> MLELLPTAVEGVSQAQITGRPEWIWLALGTALMGLGTLYFLVKGMGVSDPDAKKFYAITTLVPAIAFTMYLSMLLGYGLTMVPFGGEQNPIYWARYADWLFTTPLALLDL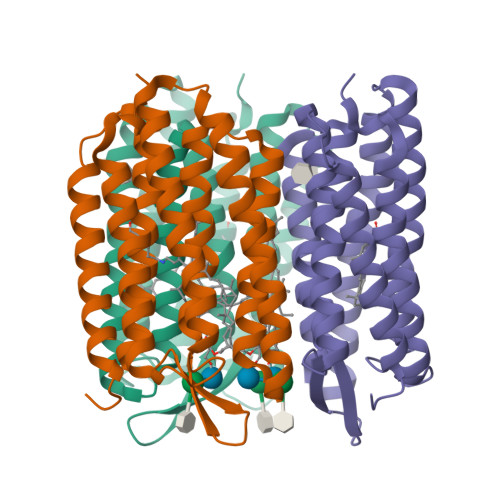ALLVDADQGTILALVGADGIMIGTGLVGALTKVYSYRFVWWAISTAAMLYILYVLFFGFTSKAESMRPEVASTFKVLRNVTVVLWSAYPVVWLIGSEGAGIVPLNIETLLFMVLDVSAKVGFGLILLRSRAIFGEAEAPEPSAGDGAAATSD>[2x]RAATVNEKLAKKKIVSIDAGRKYFSPEQLKEIIDKAKHYGYTDLHLLVGNDGLRFMLDDMSITANGKTYASDDVKRAIEKGTNDYYNDPNGNHLTESQMTDLINYAKDKGIGLIPTVNSPGHMDAILNAMKELGIQNPNFSYFGKKSARTVDLDNEQAVAFTKALIDKYAAYFAKKTEIFNIGLDEYANDATDAKGWSVLQADKYYPNEGYPVKGYEKFIAYANDLARIVKSHGLKPMAFN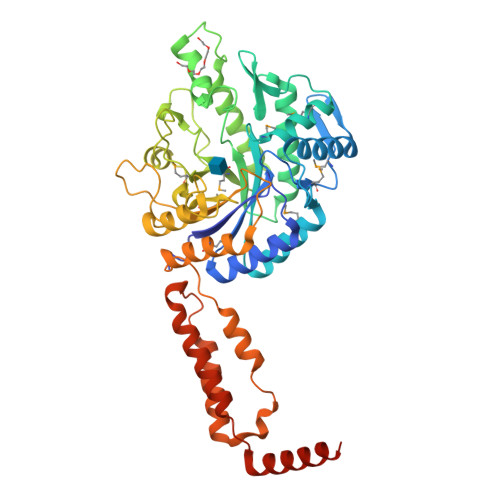DGIYYNSDTSFGSFDKDIIVSMWTGGWGGYDVASSKLLAEKGHQILNTNDAWCYVLGRNADGQGWYNLDQGLNGIKNTPITSVPKTEGADIPIIGGMVAAWADTPSARYSPSHLFKLMRHFANANAEYFAADYESAEQALNEVPKDLNRYTAESVAAVKEAEKAIRSLDSNLSRAQQDTIDQAIAKLQETVNNLTLTPEAQKEEEAKREVEKLAKNKVISIDAGRK> SNAMEVTVPATLNVLNGSDARLPCTFNSAYTVNHKQFSLNWTYQECNNCSEEMFLQFRMKIINLKLERFQDRVEFSGNPSKYDVSVMLRNVQPEDEGIYNCYIMNPPDRHRGHGKIHLQVLMEEP

Voltage-gated sodium (Nav) channels are part of membrane-embedded signaling complexes that initiate the rising phase of action potentials, a crucial event in generating and propagating electrical signals throughout the human body. As key components of these protein assemblies, β-subunits (1) modify Nav channel-gating properties; (2) regulate channel trafficking and localization to distinct surface compartments; and (3) influence channel oligomerization. Structurally, β-subunits are single-transmembrane segment glycoproteins with a short cytoplasmic C-terminal tail and a large V-type immunoglobulin (Ig) extracellular domain that may participate in homophilic and heterophilic interactions, cell adhesion, and cell migration. Of the four known β-subunits and their splice variants (β1–4; gene names Scn1b-Scn4b), β2 and β4 form a disulfide bond with an unidentified Cys within particular Nav channel isoforms.

The construct encompasses residues 30–153, and contains a single Cys mutation (C55A) to facilitate crystallization [The C55A mutation is located on the protein surface and therefore unlikely to affect the overall structure.]. The hβ2 configuration displays an Ig-like fold, consisting of eleven β-strands and three 310 helices. Other than the mutated Cys (C55A), this domain contains four additional cysteines that are arranged in two bonds. The first, intra-subunit bond, is strictly conserved among all four β-subunit isoforms and is mediated by 50Cys and 127Cys buried within the core where it links two opposing faces of the protein. The second intra-subunit bond is located within a loop that spans residues 70–77 and connects strand β5 to β6 via 72Cys - 75Cys. This loop constitutes a unique feature of hβ2 since corresponding cysteines are absent in β1, β3, and β4. The loop containing the 72Cys- 75Cys disulfide bond is modeled in a dual conformation. Of note is that the N-terminal region of hβ2 is structured rather than disordered in hβ4, adding an additional short β strand (β1) which interacts with the novel β4 strand. The hβ2 subunit possesses a corresponding Cys at position 55 that is located in a longer loop which may result in an altered spatial position of this residue when compared to hβ4.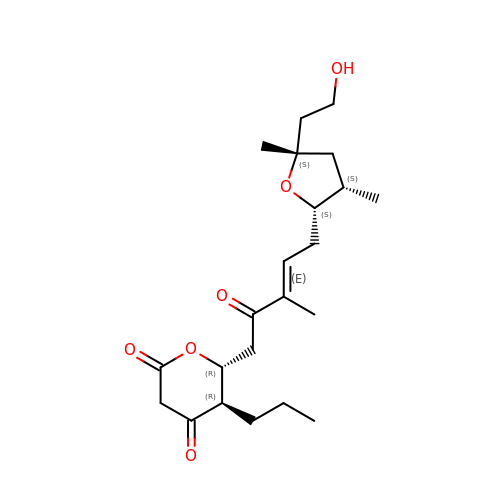(5~{R},6~{R})-6-[(~{E})-5-[(2~{S},3~{S},5~{S})-5-(2-hydroxyethyl)-3,5-dimethyl-oxolan-2-yl]-3-methyl-2-oxidanylidene-pent-3-enyl]-5-propyl-oxane-2,4-dione | C22 H34 O6 | MVJVJKSGEMISOL-KHRHQXNTSA-N>[2x]MSLLTEVETYVLSIIPSGPLKAEIAQRLEDVFAGKNTDLEVL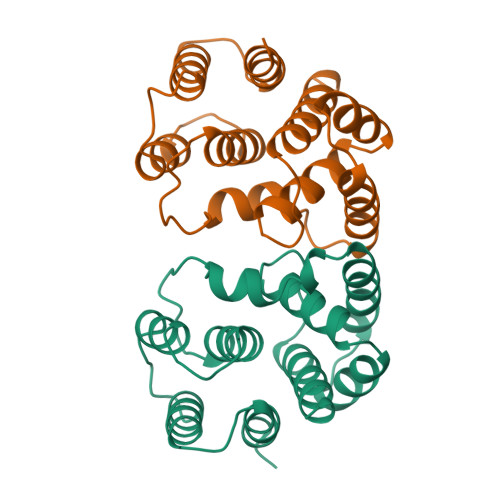MEWLKTRPILSPLTKGILGFVFTLTVPSERGLQRRRFVQNALNGNGDPNNMDKAVKLYRKLKREITFHGAKEISLSYSAGALASCMGLIYNRMGAVTTEVAFGLVCATCEQIADSQ>MIPVTELRYFADTQPAYRILKPWWDVFTDYISIVMLMIAVFGGTLQVTQDKMICLPCKWVTKDSCNDSFRGWAASSPEPTYPNSTVLPTPDTGPTGIKYDLDRHQYNYVDAVCYENRLHWFAKYFPYLVLLHTLIFLACSNFWFKFPRTSSKLEHFVSILLKCFDSPWTTRALSETVVEESDPKPAFSKMNGSMDKKSSTVSEDVEATVPMLQRTKSRIEQGIVDRSETGVLDKKEGEQAKALFEKVKKFRTHVEEGDIVYRLYMRQTIIKVIKFALIICYTVYYVHNIKFDVDCTVDIESLTGYRTYRCAHPLATLFKILASFYISLVIFYGLICMYTLWWMLRRSLKKYSFESIREESSYSDIPDVKNDFAFMLHLIDQYDPLYSKRFAVFLSEVSENKLRQLNLNNEWTLDKLRQRLTKNAQDKLELHLFMLSGIPDTVFDL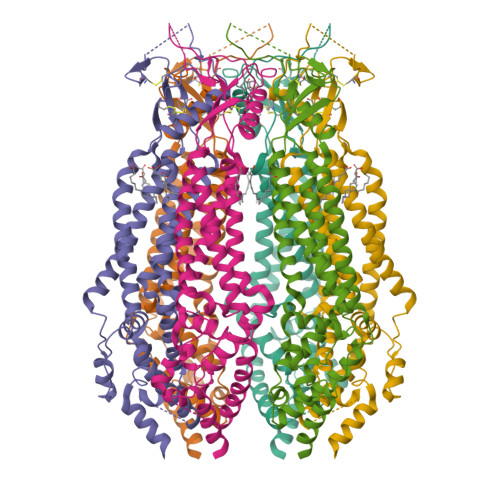VELEVLKLELIPDVTIPPSIAQLTGLKELWLYHTAAKIEAPALAFLRENLRALHIKFTDIKEIPLWIYSLKTLEELHLTGNLSAENNRYIVIDGLRELKRLKVLRLKSNLSKLPQVVTDVGVHLQKLSINNEGTKLIVLNSLKKMVNLTELELIRCDLERIPHSIFSLHNLQEIDLKDNNLKTIEEIISFQHLHRLTCLKLWYNHIAYIPIQIGNLTNLERLYLNRNKIEKIPTQLFYCRKLRYLDLSHNNLTFLPADIGLLQNLQNLAVTANRIEALPPELFQCRKLRALHLGNNVLQSLPSRVGELTNLTQIELRGNRLECLPVELGECPLLKRSGLVVEEDLFSTLPPEVKERLWRADKEQASNSLEVLFQG[6x]> MVPISPIETVPVKLKPGMDGPKVKQWPLTEEKIKALVEICTEMEKEGKISKIGPENPYNTPVFAIKKKDSTKWRKLVDFRELNKRTQDFWEVQLGIPHPAGLKKKKSVTVLDVGDAYFSVPLDEDFRKYTAFTIPSINNETPGIRYQYNVLPMGWKGSPAIFQSSMTKILEPFKKQNPDIVIYQYMDDLYVGSDLEIGQHRTKIEELRQHLLRWGLTTPDKKHQKEPPFLWMGYELHPDKWTVQPIVLPEKDS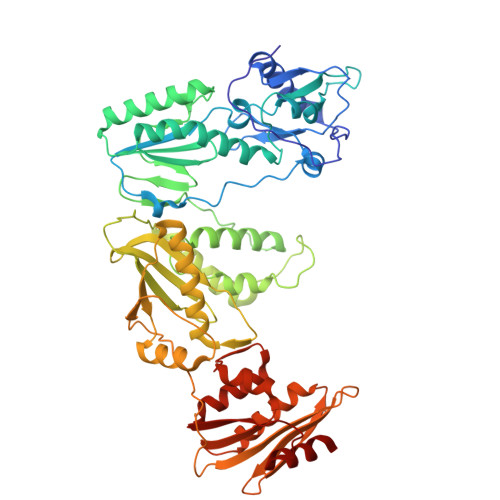WTVNDICKLVGKLNWASQIYPGIKVRQLSKLLRGTKALTEVIPLTEEAELELAENREILKEPVHGVYYDPSKDLIAEIQKQGQGQWTYQIYQEPFKNLKTGKYARMRGAHTNDVKQLTEAVQKITTESIVIWGKTPKFKLPIQKETWETWWTEYWQATWIPEWEFVNTPPLVKLWYQLEKEPIVGAETFYVDGAANRETKLGKAGYVTNKGRQKVVPLTNTTNQKTELQAIYLALQDSGLEVNIVTNSQYALGIIQAQPDKSESELVNQIIEQLIKKEKVYLAWVPAHKGIGGNEQVDKLVSA> QGMAEEVLNLQLVSVQV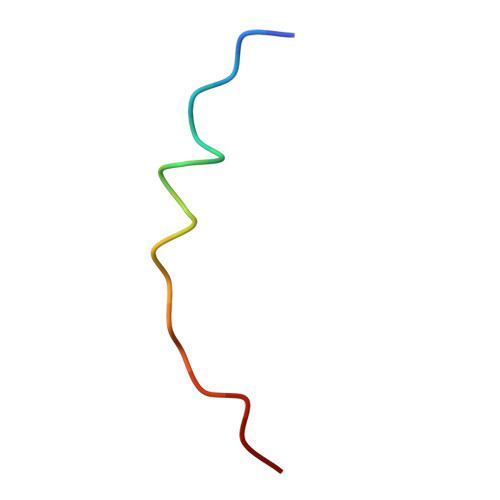D> SGRPSTDALKLCPHEEFLRLCKERAEEIYPIKERNNRTRLALIICNTEFDHLPPRNGADFDITGMKELLEGLDYSVDVEENLT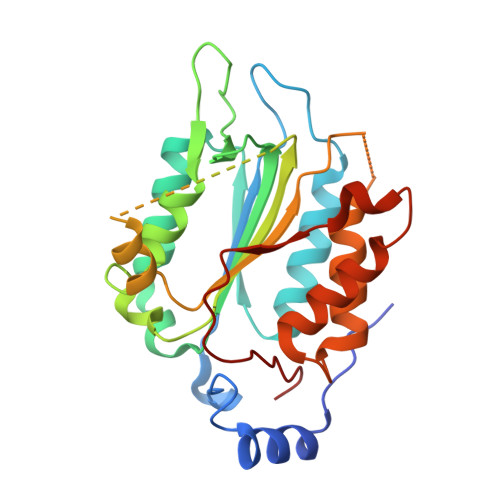ARDMESALRAFATRPEHKSSDSTFLVLMSHGILEGICGTVHDEKKPDVLLYDTIFQIFNNRNCLSLKDKPKVIIVQAARGANRGELWVRDSPASLEVASSQSSENLEEDAVYKTHVEKDFIAFCSSTPHNVSWRDSTMGSIFITQLITCFQKYSWCCHLEEVFRKVQQSFETPRAKAQMPTIERLSMTRYFYLFPGN Oxygen-free radicals formed during normal aerobic cellular metabolism attack bases in DNA and 7,8-dihydro-8-oxoguanine (8-oxoG) is one of the major lesions formed. It is amongst the most mutagenic lesions in cells because of its dual coding potential, wherein 8-oxoG(syn) can pair with an A in addition to normal base pairing of 8-oxoG(anti) with a C. Human DNA polymerase κ (Polκ) is a member of the newly discovered Y-family of DNA polymerases that possess the ability to replicate through DNA lesions. The recently discovered Y-family of DNA polymerases permit the continuity of the replication fork by allowing replication through such lesions that impede the replicative polymerases. However, whereas yeast and human Polη replicate through 8-oxoG by predominantly inserting a C, human Polκ is more efficient at inserting an A opposite the lesion than a C. In this respect, Polκ differs even from Dpo4 (its homologue in Sufolobus solfataricus) which prefers to insert a C opposite 8-oxoG. The crystal structure of Polκ in ternary complex with a template-primer DNA and an incoming nucleotide, reveals encirclement of the DNA by this unique N-terminal extension, referred to as the N-clasp.

We crystallized the Polκ catalytic core (aa 19-526) in ternary complex with a 13-nt/18-nt primer/template presenting the 8-oxoG lesion as the templating base and with dATP as the incoming nucleotide. The cocrystals diffract to 3.2 Å resolution with synchrotron radiation (Brookhaven National Laboratory) and there are two ternary complexes (A and B) in the crystallographic asymmetric unit. Polκ encircles the 8-oxoG adducted DNA in much the same way as in the ternary complex with undamaged DNA. The structure reveals an 8-oxoG(syn):A(anti) Hoogsteen base pair in the Polκ active site. The template 8-oxoG lesion is rotated to the syn conformation, wherein its Hoogsteen edge (N7 and O6) is presented for hydrogen bonding with the Watson-Crick edge of dATP (N1 and N6), which remains in the anti conformation. The C1′-C1′ distance across the 8-oxoG(syn):A(anti) Hoogsteen base pair is ∼10.96 Å, which is comparable to the distance (∼10.86 Å) in the nascent A(anti):T (anti) base pair in the ternary complex with undamaged DNA. The polymerase superimposes with an rms deviation of 0.54 Å when compared to the polymerase in the undamaged complex. The O8 of 8-oxoG (syn) is solvent exposed and does not sterically impinge on any residues in the Polκ active site. In addition, the syn conformation of 8-oxoG is stabilized by Met135 emanating from the fingers domain. A Mg2+ ion occupies a position corresponding to “metal B” in replicative polymerases, and is coordinated in the basal octahedral plane by the unesterified oxygens of dATP β- and γ-phosphates and the carboxylates of Asp107 and Asp198, and at the apical positions by the α-phosphate and the main chain carbonyl of Met108.

>MGLNDNKAGMEGLDKEKINKIIMEATKGSRFYGNELKKEKQVNQRIENMMQQKAQITSQQLRKAQLQVDRFAMELEQSRNLSNTIVHIDMDAFYAAVEMRDNPELKDKPIAVGSMSMLSTSNYHARRFGVRAAMPGFIAKRLCPQLIIVPPNFDKYRAVSKEVKEILADYDPNFMAMSLDEAYLNITKHLEERQNWPEDKRRYFIKMGSSVENDNPGKEVNKLSEHERSISPLLFEESPSDVQPPGDPFQVNFEEQNNPQILQNSVVFGTSAQEVVKEIRFRIEQKTTLTASAGIAPNTMLAKVCSDKNKPNGQYQILPNRQAVMDFIKDLPIRKVSGIGKVTEKMLKALGIITCTELYQQRALLSLLFSETSWHYFLHISLGLGSTHLTRDGERKSMSVERTFSEINKAEEQYSLCQELCSELAQDLQKERLKGRTVTIKLKNVNFEVKTRASTVSSVVSTAEEIFAIAKELLKTEIDADFPHPLRLRLMGVRISSFPNEEDRKHQQ[2x]>[4x]GAMASSVLVTQEPEIELPREPRPNEECLQILGNAEKGAKFLSDAEIIQLVN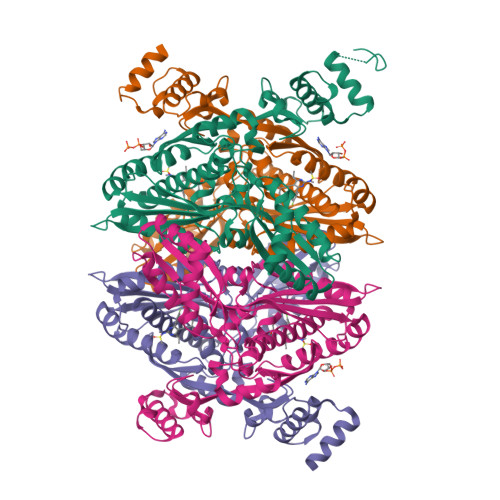AKHIPAYKLETLIETHERGVSIRRQLLSKKLSEPSSLQYLPYRDYNYSLVMGACCENVIGYMPIPVGVAGPLCLDEKEFQVPMATTEGCLVASTNRGCRAIGLGGGASSRVLADGMTRGPVVRLPRACDSAEVKAWLETSEGFAVIKEAFDSTSRFARLQKLHTSIAGRNLYIRFQSRSGDAMGMNMISKGTEKALSKLHEYFPEMQILAVSGNYCTDKKPAAINWIEGRGKSVVCEAVIPAKVVREVLKTTTEAMIEVNINKNLVGSAMAGSIGGYNAHAANIVTAIYIACGQDAAQNVGSSNCITLMEASGPTNEDLYISCTMPSIEIGTVGGGTNLLPQQACLQMLGVQGACKDNPGENARQLARIVCGTVMAGELSLMAALAAGHLVKSHMIHNRSKINLQDLQGACTKKTA We describe the approach with a detailed case study of MSS experiments on microcrystals of copper nitrite reductase from Achromobacter cycloclastes (AcNiR). Here, we describe the development of a modified MSOX approach applied to microcrystals at RT. This approach is no longer multiple structures from one crystal, but multiple serial structures from many crystals (MSS). We also describe a practical approach to separating polymorphs within a population of microcrystals and obtaining separate structures of each form, leading to two separate MSS series collected from a single batch of crystals.

A total of 20 successive images of 20 ms exposure each were measured at each aperture position of a chip, providing 20 room-temperature data sets at different dose points. Indexing of individual diffraction patterns (stills) from the first image measured from each AcNiR microcrystal revealed a bimodal distribution of unit-cell parameters. As a consequence, images were binned into two groups above and below a mid-peak cutoff of 97.25 Å, which we henceforth refer to as AcNiR-big (a = b = c = 97.75 Å) and AcNiR-small (a = b = c = 96.38 Å). Separation of the unit-cell polymorphs led to an improvement in data quality, suggesting that this analysis step is beneficial over simply merging all data regardless of unit-cell parameter. Refinement of the structure arising from each polymorph revealed two different structures, as shown in Fig. 4. The AcNiR-big and AcNiR-small structures were superimposable with an r.m.s.d. of 0.16 Å. The subsequent fall in diffracting power follows an exponential decay, with a somewhat faster fall-off with dose for the AcNiR-small population than the AcNiR-big population. The half-doses for the two polymorphs were 55 and 75 kGy, respectively. The AcNiR-small population rapidly decreases, with a concomitant increase in the population of AcNiR-big. The resulting decrease in multiplicity significantly impacts the resolution to which acceptable merging statistics are obtained. While not conclusive, this could suggest that expansion of the small cell acts as a trigger or seed leading to subsequent polymorph swapping.

> AAGAAPVDISTLPRVKVDLVKPPFVHAHDQVAKTGPRVVEFTMTIEEKKLVIDREGTEIHAMTFNGSVPGPLMVVHENDYVELRLINPDTNTLLHNIDFHAATGALGGGALTQVNPGEETTLRFKATKPGVFVYHCAPEGMVPWHVTSGMNGAIMVLPRDGLKDEKGQPLTYDKIYYVGEQDFYVPKDEAGNYKKYETPGEAYEDAVKAMRTLTPTHIVFNGAVGALTGDHALTAAVGERVLVVHSQANRDTRPHLIGGHGDYVWATGKFRNPPDLDQETWLIPGGTAGAAFYTFRQPGVYAYVNHNLIEAFELGAAGHFKVTGEWNDDLMTSVVKPASM> GLIRQQIEYKTLILNCVNPDNENSPEIPVKVLNCDTITQVKEKILDAVYKNVPYSQRPRAVDMDLEWRQGRIA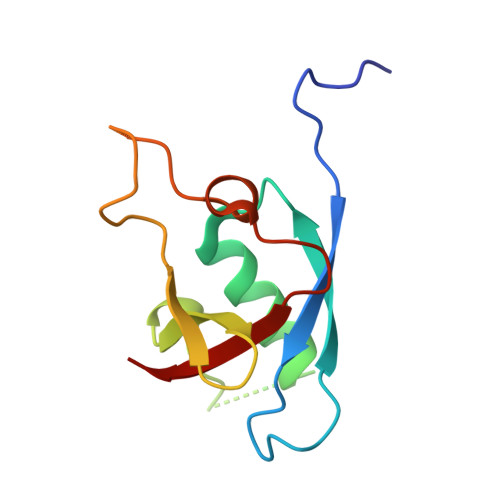RVVLQDEDITTKIEGDWKRLNTLMHYQVSDRSVVALVPK(2S)-3-{[{[(2S)-2,3-DIHYDROXYPROPYL]OXY}(HYDROXY)PHOSPHORYL]OXY}-2-[(6E)-HEXADEC-6-ENOYLOXY]PROPYL 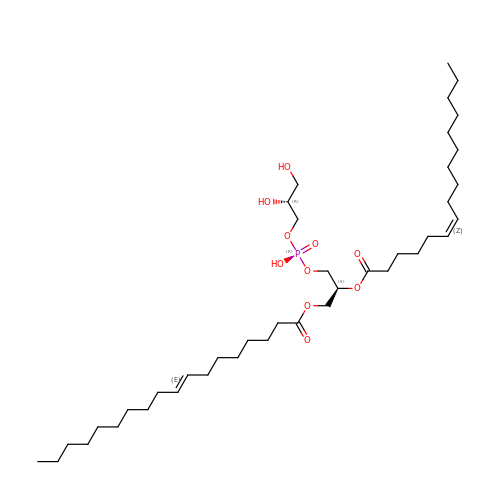(8E)-OCTADEC-8-ENOATE | C40 H75 O10 P | WLVNRDXLPAAELE-GDRYEXQRSA-N Although no X-ray crystal structure of human GBA2 is available, structures have been solved for Thermoanaerobacterium xylanolyticumTxGH116 β-glucosidase, which shares 37% amino acid sequence identity with human GBA2.8 Instead of hydrolyzing glucosylceramide like GBA2, TxGH116 exhibits high activity toward 4-nitrophenyl β-D-glucopyranoside (4NPGlc), and β-1,3- and β-1,4-linked glucooligosaccharides. The TxGH116 structure contains an N-terminal domain, formed by a two-sheet β-sandwich, tightly associated with a C-terminal (α/α)6 solenoid domain that contains the catalytic nucleophile, E441, and general acid/base, D593, residues, which were verified by chemical rescue of alanine mutants. GH116 enzymes are retaining GHs, as shown for Saccharolobus solfataricus SSO1353 β-glucosidase/β-xylosidase, human GBA2, and TxGH116.6,8,12 In the retaining mechanism, catalysis involves two carboxylic acid/carboxylate side chains with one serving as an acid/base and the other as a nucleophile. Here, we report the structures of Thermoanaerobacterium xylanolyticum β-glucosidase (TxGH116) D593N acid/base mutant in complexes with cellobiose and laminaribiose and its catalytic mechanism.

Previous work showed that the TxGH116 D593A greatly reduces enzyme activity, suggesting that D593 is the catalytic acid/base. The decreased activities were verified by kinetic analysis of D593A and D593N, which showed ∼30 000-fold decreases in the apparent kcat/Km values relative to wild-type. In all structures, the acid/base residue was mutated to asparagine (D593N) or alanine (D593A). The D593A and D593N unliganded enzymes and D593N complexes crystallized in the space group P21212, isomorphous, with wild-type TxGH116 crystals, whereas the crystals of TxGH116 D593A in complex with cellobiose and laminaribiose crystallized in the P212121 space group and had 2 molecules in one asymmetric unit. The overall structures of unliganded TxGH116 D593A and D593N, and in particular the position of amino acid residues in the active sites, were similar. However, the loops of residues 523–534 and 583–597, the last containing the mutated acid/base residue, as well as the side chains of D452 and Q727 in the active site differed from those of wild-type TxGH116. The different positions of these residues may optimize the hydrogen-bond interactions in the active sites of the acid/base mutants and reflect the flexibility of the 583–597 loop, which was shown to adopt distinct conformations in structures of wild-type TxGH116 solved in different space groups.

> AMALTGCSEKININEDKISHKIDIPDSAWTIGIGEKFKNAGHPNVKYPMIDDSYVQGAPLGGFGAGTIGRTYNGGFSRWHLEIGKNKYTTVYANQFSVFQKVEGNKDGVAQVLYAGEPENGYLSSWKWDYPKESGMYYALYPNSWYTYTNKDLPVQLAVKQFSPIIPYNYKETSYPVAVFKWTAYNPTNKNVDVSIMFTWQNMIGFFGKQVNVNSGNFNKIIKDKSKDSEIVAAVMGNISNDNEEWNGEYSIGVKKVPGVDISYKAKFVTTGDGSDLWHEFSKNGILDNKDDETPTKQDGIGSAIAVNFKLQPGQTIEVPFALSWDLPIMKFGGGDKWYKMYTKYFGKNGKNSFAILKEALNNYQKWEKMIDDWQKPILSNKSKPDWYKTALFNELYYLADGGTAWENGKVGEKDKRTNNMFGLLECFDYNYYETLDVRFYGSFPLVMLWPDIEKQVMRQFADTINVQDSSEFKVGSNGAMAVKKVQGMIPHDLGSSYALPWIKINAYDWQNPNIWKDLNSKYVLLVYRDYVLTGKTDKEFLKYTWKSVKTALDKLKEMDKDNDGIPDNEGIPDQTYATWSMKGTSAYCGSLWLAALKAAQEIGKVLKDNEAYIKYNEWYKIAQQNFEKELWNGEYYNFDTESDHKDSIMADQLAGQWYADILRLGDILPKDHVQKALKKIYEFNVMKFENGKMGAVNGMRPDGIVDESDIQAQEVWTGVTYALASFMKYRGMTEEAYNTAYGVYKMTYDKSGKGYWFRTPEAWTKDGNYRASMYMRPLSIWSMEVNYNEVLEHHHHHH>[2x]GSMEPAMEPETLEARINRATNPL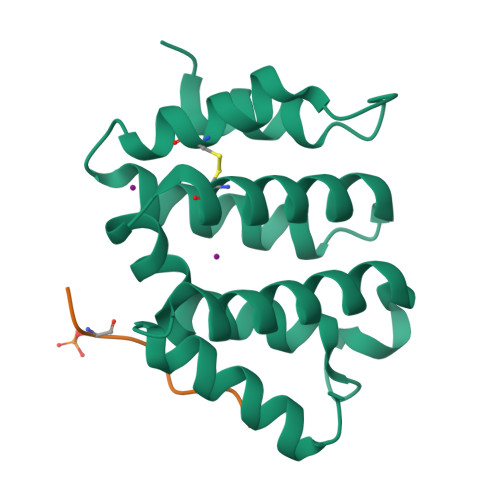NKELDWASINGFCEQLNEDFEGPPLATRLLAHKIQSPQEWEAIQALTVLETCMKSCGKRFHDEVGKFRFLNELIKVVSPKYLGSRTSEKVKNKILELLYSWTVGLPEEVKIAEAYQMLKKQGIVKS;>SGYHDDSDEDLLE[2x]>HSRAMYVYPPNVESSPELPKHIYNKLDKGQIIVVIWVIVSPNNDKQKYTLKINHDCVPEQVIAEAIRKKTRSMLLSSEQLKLCVLEYQGKYILKVCGCDEYFLEKYPLSQYKYIRSCIMLGRMPNLMLMAKESLYSQLP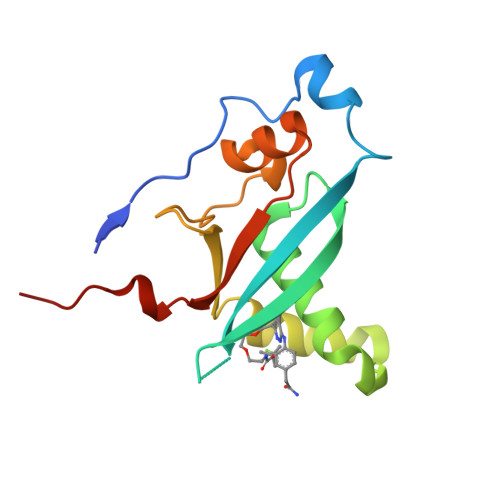MD[2x]> MAHHHHHHVGTENLYFQGFLVLIETSGNQHFIFSTNKLRENIGASELTYLATTEILFQGVDRVFQTNYYDQWSDTNSLNFLADSKLNPAIDDPKNNADIEILLATSG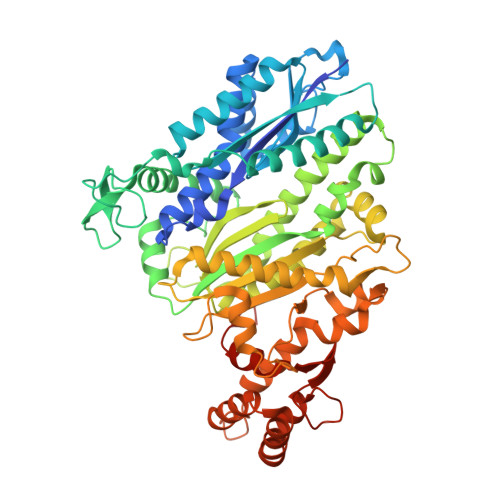KAIALVKEEGKAKQLIKEVTKQALINAPGLEIGGIYVNCNWQDKLGVAKAVKEAHKQFEVNRAKRAGANGRFLRLPIAAGCSVSELPASDFDYNADGDKIPVSTVSKVKRETAKSAKKRLRSVDGRLVNDLAQLEKSFDELDWLAVVHADGNGLGQILLSLEKYIGEQTNRNYIDKYRRLSLALDNCTINAFKMAIAVFKEDSKKIDLPIVPLILGGDDLTVICRGDYALEFTREFLEAFEGQTETHDDIKVIAQKAFGVDRLSACAGISIIKPHFPFSVAYTLAERLIKSAKEVKQKVTVTNSSPITPFPCSAIDFHILYDSSGIDFDRIREKLRPEDNTELYNRPYVVTAAENLSQAQGYEWSQAHSLQTLADRVSYLRSEDGEGKSALPSSQSHALRTALYLEKNEADAQYSLISQRYKILKNFAEDGENKSLFHLENGKYVTRFLDALDAKDFFANANHKNQGE> MSLSLLLQQHLSQPWRFLDHTSFGPTFQALQSFAYDDTLCTSIGKSQSPPTLRAWVHHNTVVLGIQDSRLPQIKAGIEALKGFQHDVIVRNSGGLAVVLDSGILNLSLVLKEEKGFSIDDGYELMYELICSMFQDHREQIEAREIVG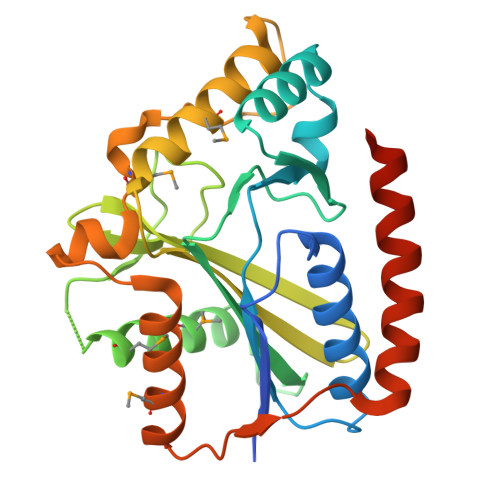SYCPGSYDLSIDGKKFAGISQRRIRGGVAVQIYLCVSGSGAERAKMIRTFYDKAVAGQPTKFVYPRIKPETMASLSELLGQPHNVSDVLLKALMTLQQHGASLLTESLSADEWLLYEQHFARISERNEKLLAEEGHHHHHH N3-PROTONATED 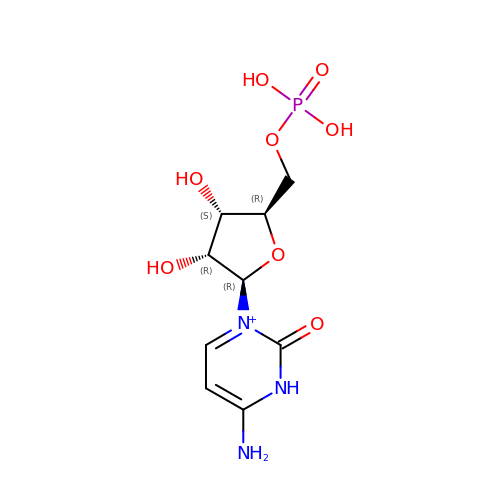CYTIDINE-5'-MONOPHOSPHATE | C9 H15 N3 O8 P | ULTJSGLMABORQB-XVFCMESISA-O> MNNDKRGLNVELSKEISKRVVEHRNRFKRLMFNRYLEFLPLLINYTNRDTVGIDFIQLESALRQNINVVVGEARNKQIMILGYVNNTYFNQAPNFSSNFNFQFQKRLTKEDIYFIVPDYLIP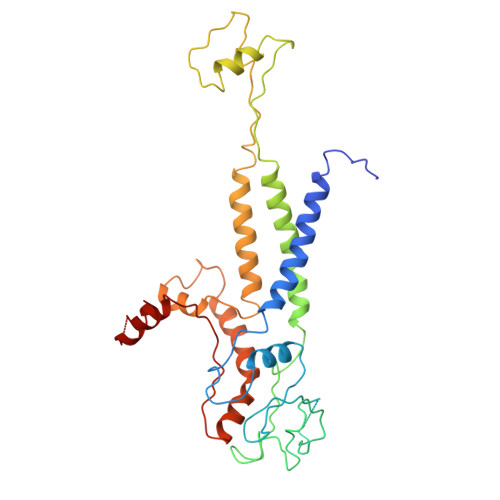DDCLQIHKLYDNCMSGNFVVMQNKPIQYNSDIEIIEHYTDELAEVALSRFSLIMQAKFSKIFKSEINDESINQLVSEIYNGAPFVKMSPMFNADDDIIDLTSNSVIPALTEMKREYQNKISELSNYLGINSLAVDKESGVSDEEAKSNRGFTTSNSNIYLKGREPITFLSKRYGLDIKPYYDDETTSKISMVDTLFKDESSDING>MRARRLVMLRHGQTDYNVGSRMQGQLDTELSELGRTQAVAAAEVLGKRQPLLIVSSDLRRAYDTAVKLGERTGLVVRVDTRLRETHLGDWQGLTHAQIDADAPGARLAWREDATWAPHGGESRVDVAARSRPLVAELVASEPEWGGADEPDRPVVLVAHGGLIAALSAALLKLPVANWPALGGMGNASWTQLSGHWAPGSDFESIRWRLD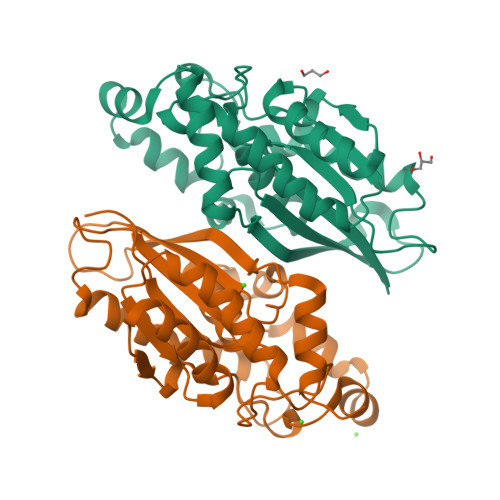VWNASAQVSSDVLKLAAALEHHHHHH[2x]>[8x]MMFGRFTERAQKVLALAQEEALRLGHNNIGTEHILLGLVREGEGIAAKALQALGLGSEKIQKEVESLIGRGQEMSQTIHYTPRAKKVIELSMDEARKLGHSYVGTEHILLGLIREGEGVAARVLNNLGVSLNKARQQVLQLLGSNETGS;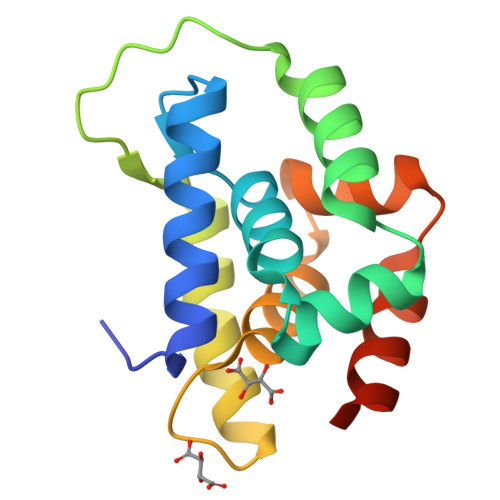>EEKEQKLQFVLRFGDFEDVISLSKLNVNGSKTTLYSFENRYYLYVDFCNMTDEEVENQLSILLEYATESSISIHRLEEYGKLIISEHALETIKKHFAS[8x]> EPSTVIMREAARHGLTIVRLQPQGSRLSLTVQ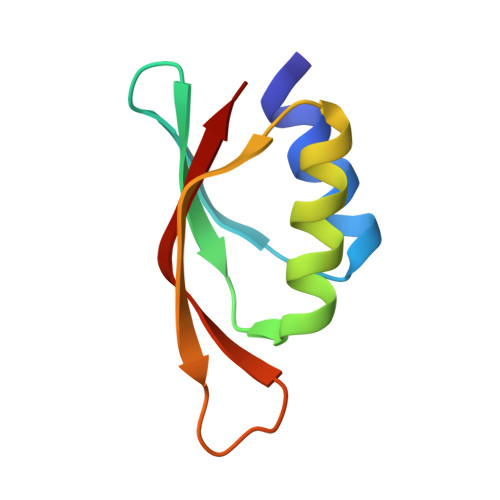PADFQALMAWLDALGQAGMTTATLAVTAVAQQPGWVTVNTLVLER>[2x]VPRGSHMKKLLVANRGEIAVRVFRACNELGLSTVAVYAREDEYSVHRFKADESYLIGQGKKPIDAYLDIDDIIRVALESGADAIHPGYGLLSENLEFATKVRAAGLVFVGPELHHLDIFGDKIKAKAAADEAKVPGIPGTNGAVDIDGALEFAKTYGYPVMIKAALGGGGRGMRVARNDAEMHDGYARAKSEAIGAFGSGEIYVEKYIENPKHIEVQILGDRHGNIIHLHERDCSVQRRNQKVIEIAPAVGLSPDFRNEICEAAVKLCKNVGYVNAGTVEFLVKDDKFYFIEVNPRVQVEHTITELITGVDIVQAQILIAQGKDLHREIGLPAQSEIPLLGSAIQCRITTEDPQNGFLPDTGKIDTYRSPGGFGIRLDVGNAYAGYEVTPYFDSLLVKVCTFANEFSDSVRKMDRVLHEFRIRGVKTNIPFLINVIANENFTSGQATTTFIDNTPSLFNFPRLRDRGTKTLHYLSMITVNGFPGIENTEKRHFEEPRQPLLNLEKKKTAKNILDEQGADAVVDYVKNTKEVLLTDTTLRDAHQSLLATRLRLQDMKGIAQAIDQGLPELFSAEMWGGATFDVAYRFLNESPWYRLRKLRKLMPNTMFQMLFRGSNAVGYQNYPDNVIEEFIRVAAHEGIDVFRIFDSLNWLPQMEKSIQAVRDNGKIAEATICYTGDILDPSRPKYNIQYYKDLAKELEATGAHILAVKDMAGLLKPQAAYRLISELKDTVDLPIHLHTHDTSGNGIITYSGATQAGVDIIDVATASLAGGTSQPSMQSIYYALEHGPRHASINVKNAEQIDHYWEDVRKYYAPFEAGITSPQTEVYMHEMPGGQYTNLKSQAAAVGLGHRFDEIKQMYRKVNMMFGDIIKVTPSSKVVGDMALFMIQNDLTEEDVYARGNELNFPESVVSFFRGDLGQPVGGFPEKLQKIIVKDKAVITDRPGLHAEKVDFETVKADLEQKIGYEPGDHEVISYIMYPQVFLDYQKMQREFGAVTLLDTPTFLHGMRLNEKIEVQIEKGKTLSIRLDEIGEPDLAGNRVLFFNLNGQRREVVINDQSVQAQVVAKRKAETGNPNQIGATMPGSVLEILVKAGDKVQKGQALMVTEAMKMETTIEAPFDGEIVDLHVVKGEAIQTQDLLIEIN

Pyruvate carboxylase (PC) is a tetrameric enzyme that contains two active sites per subunit that catalyze two consecutive reactions. A mobile domain with an attached prosthetic biotin links both reactions, an initial biotin carboxylation and the subsequent carboxyl transfer to pyruvate substrate to produce oxaloacetate. PC is mostly found as tetramers of four identical subunits, with monomers of ~120–130 kDa in size. This enzyme possesses a tetrahedral geometry with the tetramer organized in two layers. In this work, we study the structure of Lactococcus lactis PC (LlPC) during catalysis in the presence of positive allosteric regulator acetyl-CoA.

The separation of reaction steps at catalytic sites does not reveal the large conformational changes in the PC tetramer that could be coupled to the function of the enzyme. To explore the conformational space of the tetramers we performed a multibody refinement using masks enclosing dimers of BC-BC or CT-CT catalytic domains at different layers (as the bodies shown in Fig. 1c). There are only a couple of patterns related to the CT domains: showing a positive correlation of the same catalytic state when they are in the same layer; and a negative one when they are in subunits from different layers bound by their CT-CT regions. We have also observed that the PC subunits bound by their CT domains show a negative correlation in their catalytic state.>[2x]KCSLTGKWTNDLGSNMTIGAVNSRGEFTGTYTTAVTATSNEIKESPLHGTENTINKRTQPTFGFTVNWKFSESTTVFTGQCFIDRNGK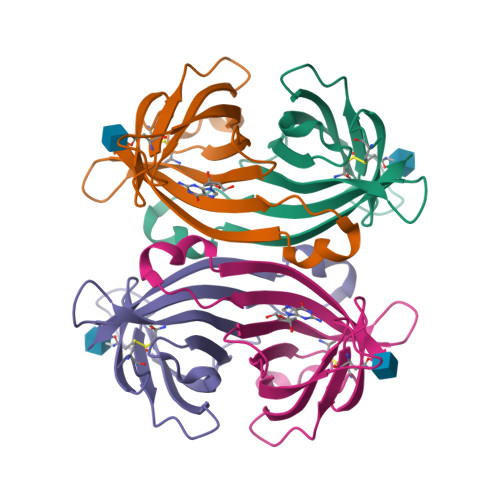EVLKTMWLLRSSVNDIGDDWKATRVGINIFTRLRTQKE>[2x]TDENLKIAIASSPAPRYITDMSIEEISREWYMLMPRQKITGGLMVKMDQAIMDKRITLKANFSVLFDQLETLVSLRAFTDDGAIVAEISPIPSMPGHSTEDVKNAIGILIGGLEWNDNSIRASENIQRFAWGIRDENGGPPLPPKQKRYMARRVESEV

During infection the influenza A virus NS1 protein participates in multiple protein-RNA and protein-protein interactions to perform a plethora of functions. The N-terminal 73 amino-acid residues of NS1 form a symmetrical homodimeric RNA-binding domain (RBD), which is connected to the central effector domain (ED; residues 86-204) via an inter-domain linker. Present models of the tertiary and quaternary structures of NS1 indicate that the protein possesses two globular domains, each capable of forming independent homodimeric interactions. Our bioinformatic analyses indicate that the N-terminal RBD forms a very stable homodimer, while the predominant and ubiquitous helix-helix contacts between C-terminal EDs bear many similarities with weak transient interfaces.

In contrast, several possible ED homodimer interfaces have been proposed based upon crystal structures obtained using NS1 proteins from various strains. While the helix-helix interface appears to be the only dimeric form of NS1 ED consistently observed in all crystal structures, it remains possible that other dimeric states (such as the strand-strand dimer) contribute to dimerization in solution. Although the helix-helix dimer interface is shared by all structures of the NS1 ED, and may have some biological role in that RNA-binding activity of NS1 is affected by its disruption, we noted that in all helix-helix structures the arrangement of the two ED monomers differs markedly relative to one another. Previous studies using recombinant Alb/76 and Ud/72 EDs have shown that a single W187A amino-acid substitution is sufficient to prevent dimerization. However, at this same concentration we routinely observe complete dimerization of the PR8 and Alb/76 NS1 EDs.> MAHHHHHHVGTDDWRCARSMHEFSAKDIDGHMVNLDKYRGFVCIVTNVASQCGKTEVNYTQLVDLHARYAECGLRILAFPCNQFGKQ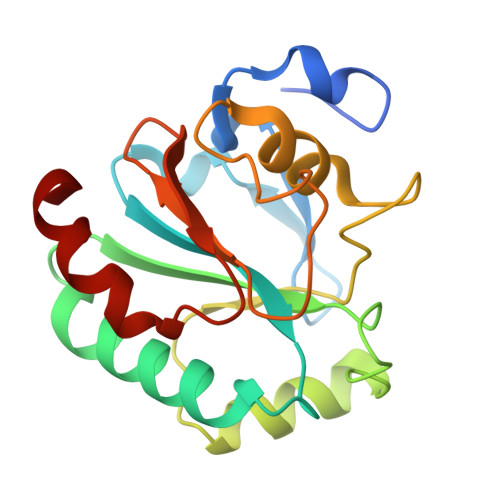EPGSNEEIKEFFAGYNFKGDLFSKICVNGDDAHPLWKWMKIQPKGKGILGNAIKWNFTKFLIDKNGCVVKRYGPMEEPLVIEKDLPHYF> LTIIT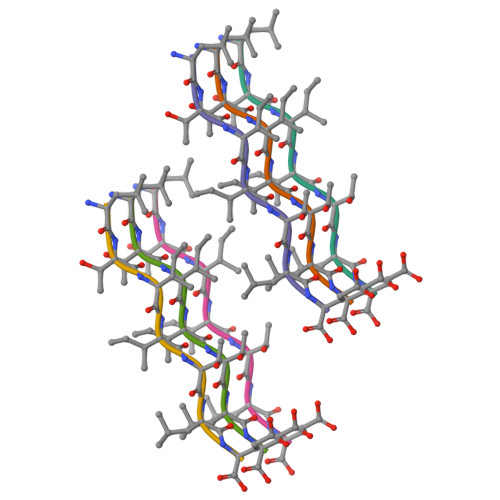LE>MDIAKWVEHARTCYSTQLDTKIKVIGVIGKDYPDHGKGDNINCYLRENVFPVAATEDETCTIRGHFSEDDQILFLVMNGVDDVANIRKCLKSNPKSNYFDAMAESECQQIRMLHFLFISCHFIIIFEQTSRIDLELMRFLKKVNSARIQLRKKINQRLVASDLRDVSFNNRILSSAESEGRMVVPRLLIAFQRNNIRPDVNPGKKLQRELYEKLEKNLDNQFSDILKLYDLIDCGASSLCQLNETIPVVHLLNPKIVKRDIIGEMFEILMADAENTKISGNAGTLPSNNSFVKFLEDNFRSEKNEISLENVIELMNCLQCVLDGDLEEKHEKTAIQTFIKRIQNDHMEEARRLYTNAQRPGERRGADRFKDSEKPVKIRSKEEHLMRFNEATHYIDSVVGVNSREALSQLQAQCNEMWQSDMRHHHHHH[3x];>MKESVRFLTDFGEISDAISDLLTSSPNFNVISAIGPQGAGKSTLLSMLAGNNSRQMYREYVFRPVSREANEQSRHQTIQIDIYIVNHQIFLDCQPMYSFSIMEGLPKVRGGRFDDSTAMSDTLRLTAFLLYVSHTVLVVSETHYDKVIIDTLRVAEQIRPYLAIFRPKLAIDRKTNLVFIKTKASSIDLAPTVIREREELLRLSFQDSRWLKVSQEPFKTLIVLEEIRVRREHLFEEGDEPDEAASLNEFDEQIAELREELQKNREDFTVETAAMDEKKWLDMCREVIRDKTLHKTLKEYQRAMTDGVRTHFDNGFH[3x]

The SMG1 kinase is an essential NMD factor in metazoans and is associated with two recently identified and yet poorly characterized proteins, SMG8 and SMG9. We found that SMG8–SMG9 is a G-domain heterodimer with architectural similarities to the dynamin-like family of GTPases such as Atlastin and GBP1. SMG8 and SMG9 interact with each other and inhibit the kinase activity of SMG1 in vitro. Nucleotide binding occurs at the G domain of SMG9 but not of SMG8.

We proceeded to obtain the structure of a nucleotide-bound SMG8c–SMG9c complex. Although the SMG8c–SMG9c crystals cracked when soaking GTP, GDP soaking experiments were successful. Diffraction data to 2.65 Å resolution showed the presence of well-defined electron density for a GDP moiety in SMG9c but not in SMG8c. GDP binds SMG9c at a similar position as in Atlastin and GBP1, in particular with similarities at the phosphate-binding loops, e.g., at the motifs G1 (P loop), G2 (switch 1), and G3 (switch 2). In SMG9c, the P loop residues Lys99SMG9 and Ser100SMG9 coordinate the phosphates of GDP. Although parts of the switch regions are disordered in our GDP-bound structure, the switch 2 residue Asp150SMG9 is at the position expected for coordinating the magnesium ion, while the switch 1 residue Thr135SMG9 is 10 Å away from the position expected upon γ-phosphate binding. First, there is a conserved proline residue (Pro153SMG9, disordered in the present structure) at the position of switch 2 typically occupied by a glycine. Second, there is a conserved glycine residue (Gly96SMG9) in the P loop at the equivalent position of the so-called arginine “finger” (Arg77Atlastin). At the corresponding position of Asp218Atlastin, SMG9 features a conserved lysine residue (Lys241SMG9) that stacks with its aliphatic portion on top of the guanine base. Fitting the GDP-bound SMG8–SMG9 structure in EM densities of the human SMG1–SMG8–SMG9 complex raises the possibility that the nucleotide site of SMG9 faces SMG1 and could impact the kinase conformation and/or regulation.In all living cells the signal recognition particle (SRP) recognizes nascent polypeptides destined for secretion or membrane insertion as they emerge from translating ribosomes. As SRP binds to signal sequences emerging from the ribosomes, the resulting complex composed of the SRP and the ribosome-nascent chain complex is then targeted towards the membrane through the GTP-dependent interaction with the membrane-associated SRP receptor (SR also named FtsY in bacteria). We describe the X-ray structures of SRP54 and SRP19 the two protein constituting the proteinaceous core of the SRP from the hyperthermophilic archaeon Pyrococcus furiosus. SRP54 and SRP19 constitute the conserved core in all archaeal and eukaryotic SRPs.

We solved two distinct crystal forms of Pfu-SRP19. Two molecules of SRP19 associate in a dimer with an extended β-sheet surface built around the anti-parallel association of their respective β2 strands. Observation of the crystal packing in the orthorhombic subunit reveals a tetrameric arrangement between symmetry-related molecules that is similar to the one observed in the monoclinic form. Pfu-SRP19 is characterized by a more extended β-sheet due to longer β2 and β3 strands when compared with all other available SRP19 structures. The structure is also characterized by two loops (L1 and L2). The loop L1, the primary RNA-binding surface is rigid and well defined in density whereas the loop L2 is disordered and absent in our final models. Superposition of our free SRP19 structure on the RNA-bound SRP19 structures reveals that the difference between free SRP19 and the RNA-bound forms lies exclusively in the conformation of the L2 loop region. The disordered L2 region of the “free” protein has a well-defined conformation in the RNA bound structures. In contrast the L1 loop remains structurally unchanged, this is observed even when all available structures of free and RNA-bound SRP19 from different species are compared. Through an induced fit mechanism involving the rearrangement of its disordered L2 loop, SRP19 assists proper folding of the SRP RNA and therefore favors subsequent binding of SRP54.

>[2x]MGRFVVWPSELDSRLSRKYGRIVPRSIAVESPRVEEIVRAAEELKFKVIRVEEDKLNPRLSGIDEELRTFGMIVLESPYGKSKSLKLIAQKIREFRRRSAGTLVPR>MAYLNRDQRREMILQAAMQIALAEGFTAMTVRRIATEAQTSTGQVHHHFSSASHLKAEAFLKLMEQLDEIEQTLQTTSQFQRLFILLGAENIDRLQPYLRLWNEAELLIEQDIEIQKAYNLAMQSWHQAIVQSIECGQKEGEFKNRSNSTDIAWRLIAFVCGLEGIYKLGLQGLAEEDFKRHTEAIIRLELL[2x]

The polyamine-binding protein AmvR regulates the multidrug efflux pump AmvA, which is pivotal for transporting polyamines, an abundant and prevalent class of amino acid-derived metabolites. AmvA abundance in vivo is transcriptionally regulated by AmvR, a TetR/AcrR-like regulator that senses cellular polyamine levels and enables the dynamic modulation of amvA expression in response to fluctuating growth conditions. The overall fold change observed in AmvR is characteristic of the TetR/AcrR family of transcription factors and consists of an all-helical regulatory domain (α1–α9). The AmvR protein can be further divided into two subdomains in each protomer: the N-terminal DNA-binding domain (DBD) and the C-terminal ligand-binding domain (LBD).

We successfully determined the crystal structure of AmvR complexed with spermidine to precisely investigate the substrate-binding pocket. Two AmvR polypeptide chains were situated within the asymmetric unit of the crystal and formed a homodimer. The high-resolution structure indicated that the stoichiometry of spermidine binding to AmvR was a 1:1 ratio (one molecule of spermidine present in each protomer of AmvR). However, the overall structure of this TetR family regulator remains largely unchanged between the apo and SPD-bound states, unlike other regulators that exhibit substantial structural differences. Notable alterations were observed only in α4 and α6 of the LBD subdomain. The α4 undergoes a movement of approximately 2.8 Å to create sufficient space for ligand binding, and the α6 also moves to enhance compactness. The ligand-binding pocket consists of the residues in α4, α6–8, and loops between α5 and α6, which form a long narrow tunnel. The side chain of E164 and N103 in the α4 helix, along with the side chain of E106 in the α6 helix, moved to form hydrogen bonds with the amine group of spermidine. Another amino group of spermidine formed a hydrogen bond with the side chain of E71, which underwent movement along the α6 helix and the carbonyl group on the main chain of L86. The hydrophobic interactions provided by W102, W126, and L99 are also crucial for spermidine binding, especially W102 at α6, which shifts and stabilizes spermidine.>MRIDTVNVLLEALPYIKEFYGKTFVIKFGGSAMKQENAKKAFIQDIILLKYTGIKPIIVHGGGPAISQMMKDLGIEPVFKNGHRVTDEKTMEIVEMVLVGKINKEIVMNLNLHGGRAVGICGKDSKLIVAEKETKHGDIGYVGKVKKVNPEILHALIENDYIPVIAPVGIGEDGHSYNINADTAA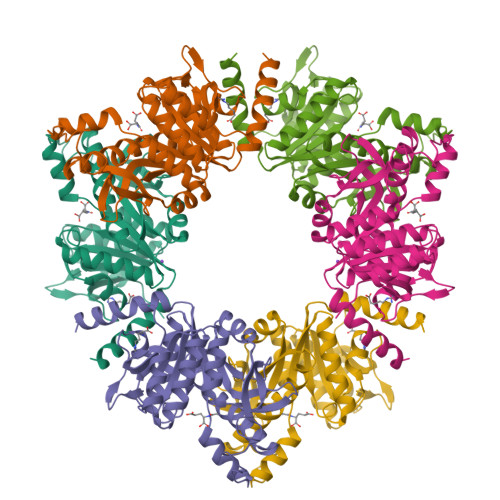AEIAKSLMAEKLILLTDVDGVLKDGKLISTLTPDEAEELIRDGTVTGGMIPKVECAVSAVRGGVGAVHIINGGLEHAILLEIFSRKGIGTMIKELEG[3x]> MHHHHHHMVEVKKHKFPGVYVVIDDDGSEKIATKNLVPGQRVYGERVIKWEGEEYRIWNPHRSKLGAAIVNGLKNFPI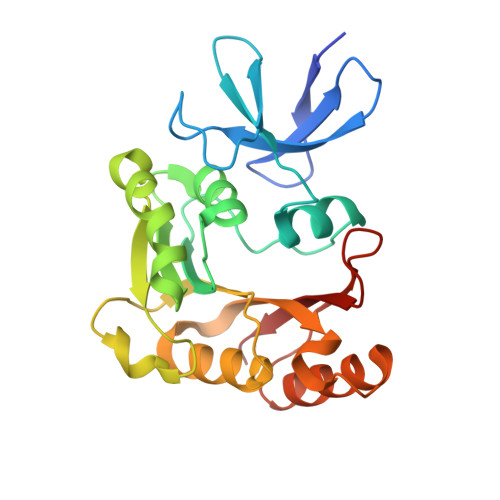KPGKSVLYLGIASGTTASHVSDIVGWEGKIYGIEFSPRVLRELVPIVEERRNIIPILGDATKPEEYRALVTKVDVIFEDVAQPTQAKILIDNAKAYLKRGGYGMIAVKSRSIDVTKEPEQVFKEVERELSEYFEVIERLNLEPYEKDHALFVVRKP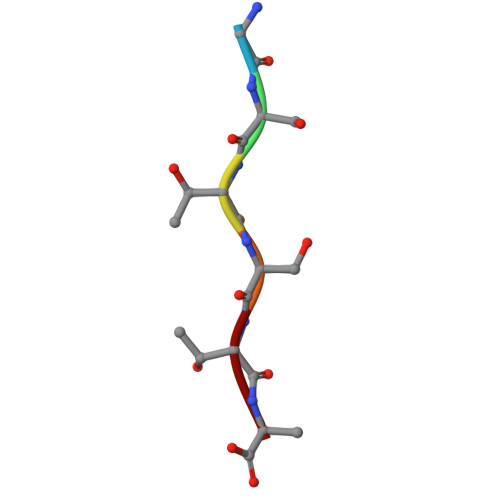> GSTSTA6-{[(3R,4R)-4-{[(3E)-4-(3-fluorophenyl)but-3-en-1-yl]oxy}pyrrolidin-3-yl]methyl}-4-methylpyridin-2-amine 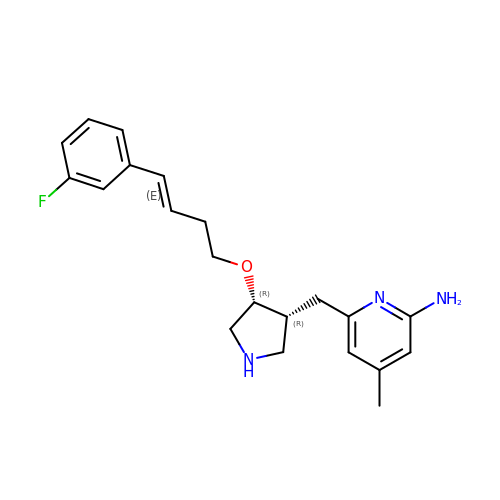| C21 H26 F N3 O | GKGVFZUGOXZFKN-YUOLOVIMSA-N Bdellovibrio bacteriovorus is a bacterium that preys upon a wide range of other Gram-negative bacteria, entering their periplasm and consuming them from within. Proteomic and structural analyses of vesicle contents reveal several fibre-like proteins, which we name the mosaic adhesive trimer (MAT) superfamily, and show localization on the predator surface before prey encounter. Structural studies reveal a variety of domain usages (and therefore binding capabilities) at the fibre C-termini, placing these on intertwined trimeric β-prisms. Using independent but complementary approaches, we identified and characterized a MAT superfamily of trimeric fibre proteins with diverse adhesive tips, able to fulfil the long-sought-after role of multiplicity of molecular recognition and handling of diverse epitopes (across a wide prey range), by the bacterial predator B. bacteriovorus.

A C-terminal region (amino acids 632–922) of Bd3182 confirmed the predicted chaperone and protease activity of the S74 domain, yielding the expected two bands, with self-cleavage at catalytic residue S782. We generated three different forms of the mature ‘tip’ region of family member Bd3182 (we describe the 1.1 Å form herein). Each face of the β-helix is formed from multiple chains, resulting in an intertwined structure. The RMSDs indicate that Bd3182 is a true S74 member, with a surface cleft similar to that of others, whose exposure (via S74 proteolysis) is necessary to bind their O-antigen ligand. An AlphaFold18 model of full-length Bd3182 reveals that trimerization is retained along its entirety, generating a fibre ~550 Å long. Thus, predatory bacterial MAT protein Bd3182 is related to phage adhesins but uses a distinctly longer fold with a more exposed binding cleft.

>GGTNDAFSLSFETNNTPRMTIDDVGRVGVGTTAPTSALHVIGTGEVARFVTSATGGVVIDSTALNYNPSLIYRKTNINRWSMMVNAASETGGNAGSNLSILRYDDTGATLGAAVTIDRASGFFGINTAAPAYNIHVTGTAGLSTGSAWTVAS[6x]> MHHHHHHMSTTVEKIKAIEDEMARTQKNKATSFHLGQLKAKLAKLRRELLTSASSGSGGGAGIGFDVARTGVASVGFVGFPSVGKSTLLSKLTGTESEAAEYEFTTLVTVPGVIRYKGAKIQMLDLPGIIDGAKDGRGRGKQVIAVARTCNLLFIILDVNKPLHHKQIIEKELEGVGIRLNKTPPDILIKKKEKGGISITNTVPLTHLGNDEIRAVMSEYRINSAEIAFRCDATVDDLID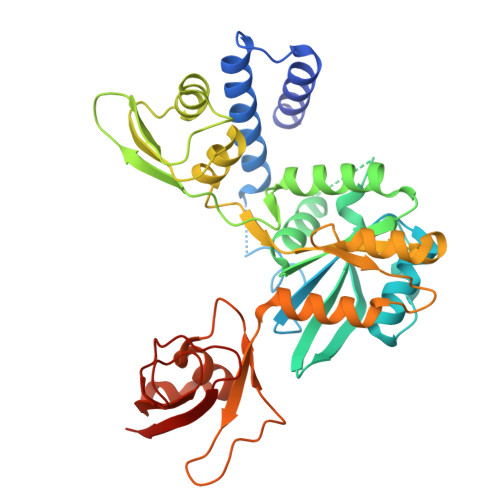VLEASSRRYMPAIYVLNKIDSLSIEELELLYRIPNAVPISSGQDWNLDELLQVMWDRLNLVRIYTKPKGQIPDFTDPVVLRSDRCSVKDFCNQIHKSLVDDFRNALVYGSSVKHQPQYVGLSHILEDEDVVTILKK> LENKPRIPVVWIHGLECTGCTESFIRSAHPLAKDVILSLISLDYDDTLMAAAGTQAEEVFEDIITQYNGKYILAVEGNPPLGEQGMFCISSGRPFIEKLKRAAAGASAIIAWGTCASWGCVQAARPNPTQATPIDKVITDKPIIKVPGCPPIPDVMSAIITYMVTFDRLPDVDRMGRPLMFYGQRIHDKCYRR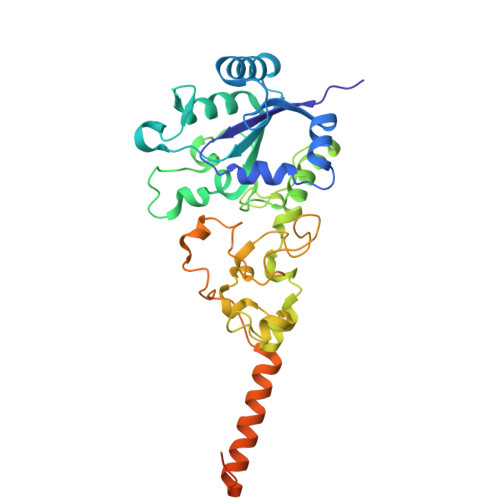AHFDAGEFVQSWDDDAARKGYCLYKMGCKGPTTYNACSSTRWNDGVSFPIQSGHGCLGCAENGFWDRGSFYSRVVDIPQMGTHSTADTVGLTALGVVAAAVGVHAVASAVDQRRRHNQQPTETEHQPGNEDKQARSHHHHHH> SGIVPTLQNIVATVTLGCRLDLKTVALHARNAEYNPKRFAAVIMRIREPKTTALIFASGKMVVTGAKSEDDSKLASRKYARIIQKIGFAAKFTDFKIQNIVGSCDVKFPIRLEGLAFSHGTFSSYEPELFPGLIYRMVKPKIVLLIFVSGKIVLTGAKQREEIYQAF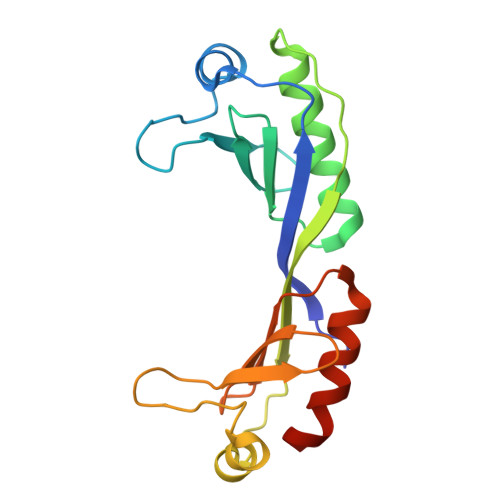EAIYPVLSEFRKM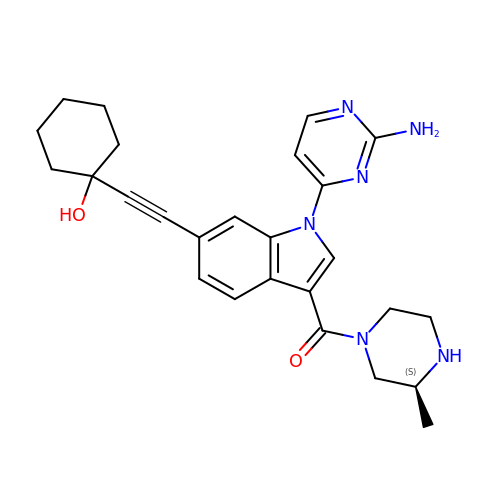[1-(2-azanylpyrimidin-4-yl)-6-[2-(1-oxidanylcyclohexyl)ethynyl]indol-3-yl]-[(3S)-3-methylpiperazin-1-yl]methanone | C26 H30 N6 O2 | SYJOLNGRHPSSMR-SFHVURJKSA-N>[2x]GWVSGQLRYSVVEESEPGTLVGNVAQDLGLKGTDLLSRRLRLGSE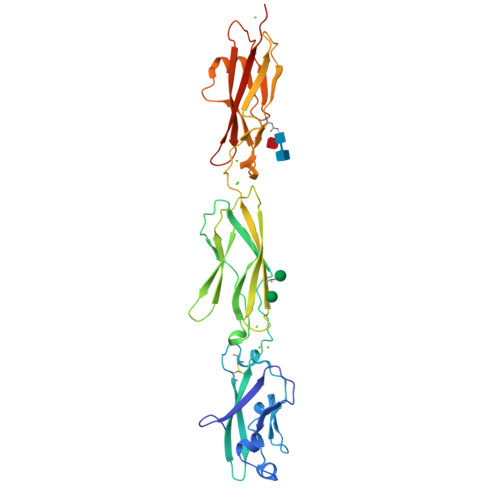ENGRYFSLSLVSGALAVSQKIDRESLCGASTSCLLPVQVVTEHPLELTRVEVEILDLNDNSPSFATPDREMRISESAAPGARFPLDSAQDPDVGTNTVSFYTLSPNSHFSLHVKTLKDGKLFPELVLEQQLDRETQARHQLVLTAVDGGTPARSGTSLISVIVLDVNDNAPTFQSSVLRVGLPENTPPGTLLLRLNATDPDEGTNGQLDYSFGDHTSETVKNLFGLDPSSGAIHVLGPVDFEESNFYEIHARARDQGQPAMEGHCVIQVDVGDANDHHHHHHHH>[2x]GSMSLFPGDIEELARRIITDFTPLGLMVSTAESCTGGLIAGALTEIAGSSAVVDRGFVTYTND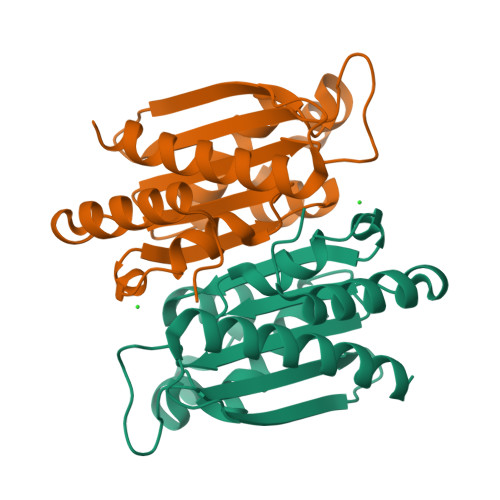AKRDMLGVGTETLTTFGAVSRQTALQMAHGALYRSRANFAVAVTGIAGPGGGSAEKPVGLVHLATKARNGNVLHHEMRYGDIGRTEIRLATVRTALEMLIALNQAGSV>XGEIAQALKEIAKAAKEIAWALKEIAQALKGX[6x]

αHBs are oligomers of 5 or more α-helical peptides that assemble into coiled-coil structures with central solvent-accessible channels. We targeted two properties of αHBs: oligomeric state, which directly affects the internal diameter of the channel; and the identities of channel-facing residues, which fine tune this dimension and introduce different chemistries. The αHBs are loaded with an environment sensitive dye (in this case, 1,6-diphenyl-1,3,5-hexatriene, DPH) that binds within the channels and fluoresces. Accordingly, challenging the array with analytes leads to differential displacement of the dye across the array to give a fluorescent fingerprint.

Despite the requirements for aliphatic residues at a and d, up to 40% of these can be changed to other side chains without compromising barrel integrity. We introduced mutations at one or two of these sites to generate four groups of αHB: Group I had entirely hydrophobic interiors, but with different sizes and shapes of channel; Groups II and III had polar uncharged or polar charged residues, respectively, at specific points along the channel; and Group IV had aromatic residues installed in their channels. In detail, the sixteen Group I peptides included: previous designs for a pentamer, 3 hexamers, 2 heptamers and an octamer all verified by X-ray crystallography;27,29 single and/or double mutations to Ala and Gly at central a and d sites to generate larger channels; a single-Pro mutant at the final d site to kink and open the C-terminal end of the channel; and a variant with all a sites made Met to vary the hydrophobic chemistry used. Finally, one third of the designs were crystallized and yielded 12 X-ray crystal structures, all of which were open αHBs with fully accessible channels. Conversely, the FAs generate signal through interactions with the more-hydrophobic and aromatic-containing channels (Group I and IV).We recently identified PbdA, a P450 from Rhodococcus jostii RHA1, and PbdB, its cognate reductase, which catalyze the O-demethylation of para-methoxylated benzoates (p-MBAs) to initiate growth of RHA1 on these compounds. PbdA is a member of the CYP199A family, which appears to have evolved to O-demethylate p-MBAs. Atomic-resolution structures of PbdA in complex with p-MBA, p-ethylbenzoate, and veratrate revealed a cluster of three residues that form hydrogen bonds with the substrates’ carboxylate: Ser87, Ser237, and Arg84. Similar to the substrate-bound structures of CYP199A2 and CYP1994, all three structures were in a closed conformation, with the F and G helices occluding the substrate access channel.

PbdA also catalyzed the hydroxylation and dehydrogenation of p-ethylbenzoate even though RHA1 did not grow on this compound. To investigate how widespread these activities are in the CYP199A subfamily, we characterized the ability of PbdA to bind and transform p-EB. PbdA bound p-EB with close to the same affinity as p-MBA, its preferred substrate. The transformation of p-EB by PbdAB was remarkably well-coupled to NADH consumption. Moreover, the apparent kcat/KM of PbdAB for p-EB was within 50% that for p-MBA. Finally, we analyzed the products of p-EB oxidation by RHA1 resting cells induced to express the PbdAB system. Both desaturation and hydroxylation products were detected, along with acetyl and epoxide derivatives presumably produced through secondary oxidation of the desaturation product. Despite the efficient oxidation of p-EB by PbdAB, RHA1 did not grow on this compound. PbdAB also efficiently catalyzed the hydroxylation and desaturation of p-EB, as reported in CYP199A4 (21). However, derivatives of Pseudomonas sp. B13 were evolved to utilize p-EB as a sole substrate via meta-cleavage, overcoming both regulation and enzyme inhibition, both of which are bottlenecks in its degradation by the WT strain. It is therefore likely that the high affinity and specificity of PbdA for p-EB reflect its chemical similarity to p-MBA and this is not a physiologically relevant reaction.

>[2x]MGSSHHHHHSSGENLYFQGHMFAPAPALPVSDADPFALDVLQDPLPFQANLRDAGPVVYLRRYDVFALGRYEQVHAALTDWQSFQSAAGVGLSNFRYETPWRPPSILLEADPPHHDAPRAVLSKILGPRALQKLRAAWIQDAEALVDQLLANTTEFDAVTDLAAAFPLRVFPDAVGIPDAGRENLLPYGDHAFNAFGPANGLVEKGAPRVAELSGWVNAQCARDALTGDGFGAQIWAAADRGDITYEQAPLVVRSLLTAGVDTTVNGLAAVLYAFATHPDQWARLRENRTLARTAFDEAVRWESPVQTFFRTATRDTEIGGATIPDGKKILMFLGAANRDPRRWENPEVFDLGRNPSGHVGYGMGIHQCVGQHVARLESEALLTALASRVHSLEIAGPVHRHLNNTLRSWESVPVKVRLP>[8x]MATETNYPVPYRSKLTEPFEPGQTLIIKGKTAEDSVRFTINLHNTSADFSGNDVPLHISVRFDEGKIVFNTFSKGEFGKEERKSNPYKKGDDIDIRIRAHDSKFSISVDQKEVKEYEHRVPLSSVTHFSVDGDILITYIHWGGKYYPVPYESGLAGDGLAPGKSLLIFATPEKKGKRFHINLLKKNGDIALHFNPRFDEKAIVRNSLISGEFGN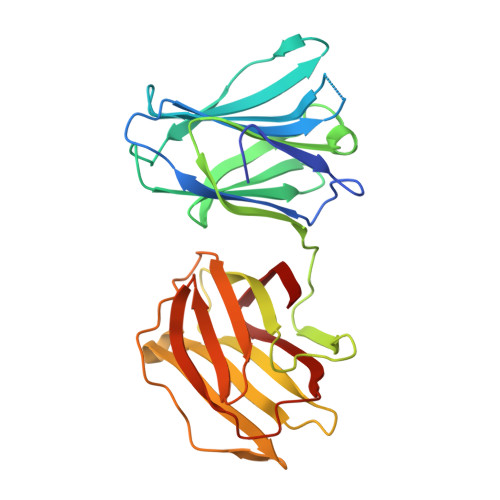EEREGKNPLEKGIGCDLEFRNEEYAFQIYVDGERFATYAHRLDPHDINGLQIGGDVEVTGIQMV(2~{R},3~{S},4~{S},5~{R},6~{R})-2-(hydroxymethyl)-6-[[(3~{S},5~{R},8~{R},9~{R},10~{R},12~{R},13~{R},14~{R},17~{S})-17-[(2~{S})-2-[(2~{S},3~{R},4~{S},5~{S},6~{R})-6-(hydroxymethyl)-3,4,5-tris(oxidanyl)oxan-2-yl]oxy-6-methyl-hept-5-en-2-yl]-4,4,8,10,14-pentamethyl-12-oxidanyl-2,3,5,6,7,9,11,12,13,15,16,17-dodecahydro-1~{H}-cyclopenta[a]phenanthren-3-yl]oxy]oxane-3,4,5-triol | C42 H72 O13 | 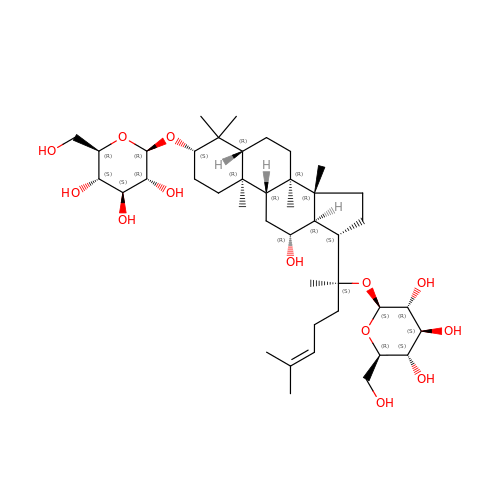SWIROVJVGRGSPO-JBVRGBGGSA-N> GSRNKHHSPKRHSQTSFPAQKSTPQSQQLTSTTPQSQQQEASERSESQQIMFLSEPFVRTALVKGSFKTIVQLPKYVDLGEWIALNVFEFFTNLNQFYGVVAEYVTPDAYPTMNAGPHTDYLWLDANNRQVSLPASQYIDLALTWINNKVNDKNLFPTKNGLPFPQQFSRDVQRIMVQMF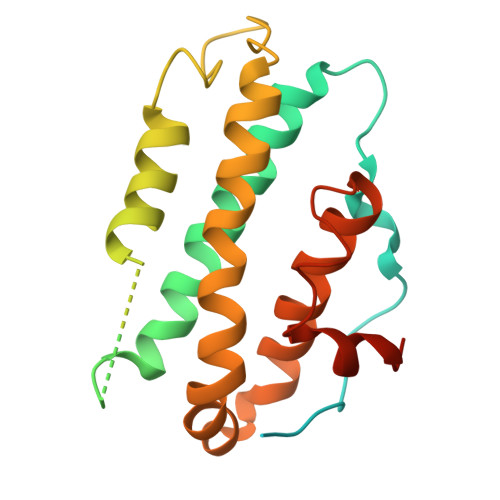RIFAHIYHHHFDKIVHLSLEAHWNSFFSHFISFAKEFKIIDRKEMAPLLPLIESFEKQGKIIYN>[2x]MGDTKEQRILRYVQQHAKP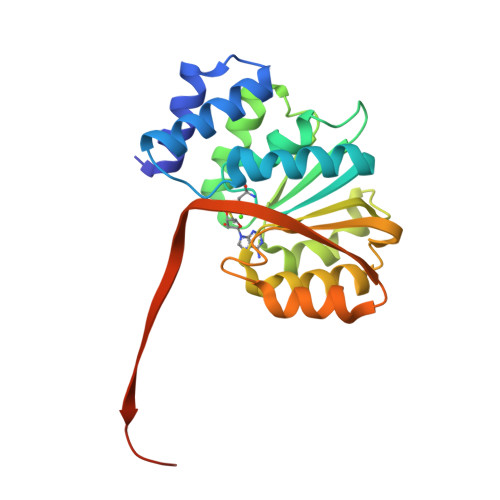GDPQSVLEAIDTYCTQKEWAMNVGDAKGQIMDEVIQEHNPSLVLELGAYCGYSAVRMARLLSPGARLLTMEKNPDYAAITQQMLNFAGLQDKVTILIGASQDLIPQLKKYDVDTLDLVFLDHWKDRYLPDTILLEECGLLRKGTVLLADNVIVPGTPDFLAYVRGSSSFECTHYSSYLEYMKVVDGLEKAVYKGPSSPKQPLEHHHHHH> MTKQEKTALNMARFIRSQTLTLLEKLNEL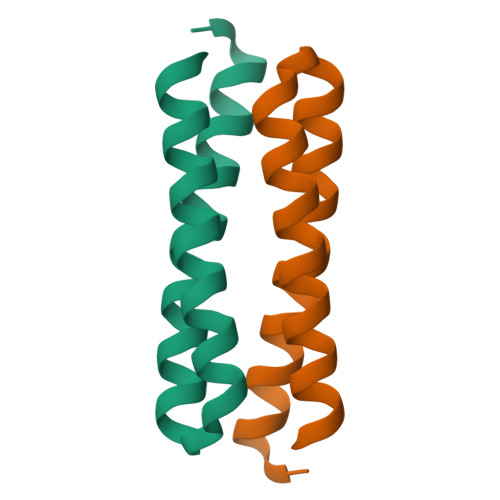DADEQADICESLHDHADELYRSCLARFGDDGENL> MYLIICYIYIYIYXXIFIRRCLLQPRHLMFRFFSLRLAPAPSADAAAKLPAGKPANK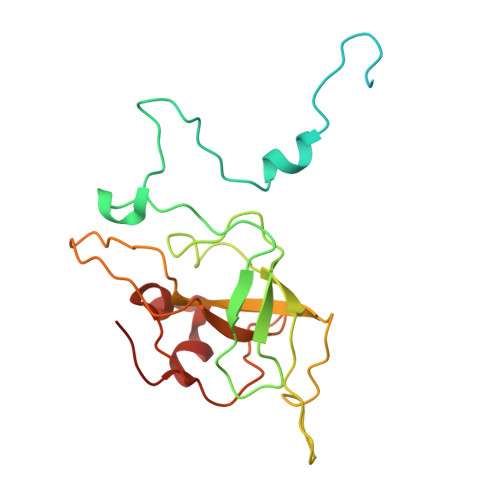SWFRHNLIIRRKASYRSRWGTGAEGYGTGVPFSDQVKLHCVDNTNCKHVRLISKATAERFAHCRVFPAVAHRVSVQRFKSGRGEVSRHRVKPGNIYWVCLLSRRQTNTRMSGLRTNFDRNTCILMNDQRVPLGTRVMYCAGRHVNHKYHLKAVVLANFFV> MTQNIKNLDLSIELDKKMYKKKLKVLQYEMLNAQQFLLKNKIGLILVFEGMDAAGKGGAIKRLIERVDPRGYVVHPISAPQPHELRYNYLQRFWRKLPQHGQIAVFDRSWYGRVLVERIEGFATKDEWSRAYEEINNFEKILTAGDYIIIKFWLHVSDEEQLKRFKEREQNPYKSWKLTDEDWRNREKSPQYIEAANEMFE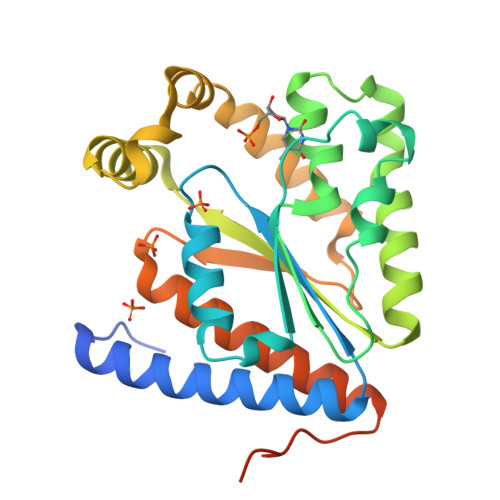KTDKKNAPWVLVAGNDKKYARVQVLQETLAHIEREALKRGLHLTNVLDKAHLEDAESSSLDILNEKKK>[4x]KVKRDISAFQKVIQDISLAVNKFNVDIERYVGGDASHLLADGNVLIKATLDGVQSLQNEPPLSSMEALALVGPVQDLSNQILLAIQNLIDKKEPLVQAGFGGKVENNLRQQEE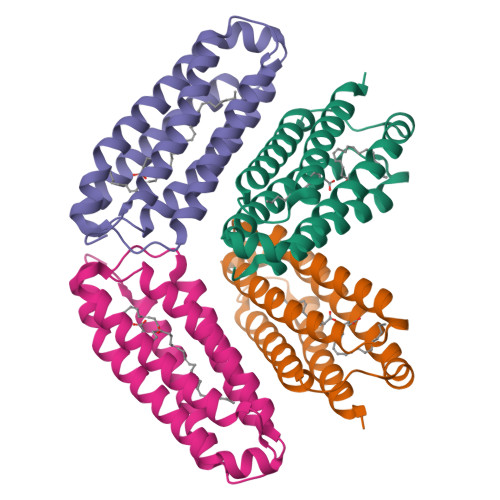AAQKLSELVSTKVPHELADISRQLSDGIAAGIKKGIDAFAGT>MEKTRPDYTSFNTVDEWLEAIKMGQYKESFANAGFTSFDVVSQMMMEDILRVGVTLAGHQKKILNSIQVMRAQMNQIQSVEV[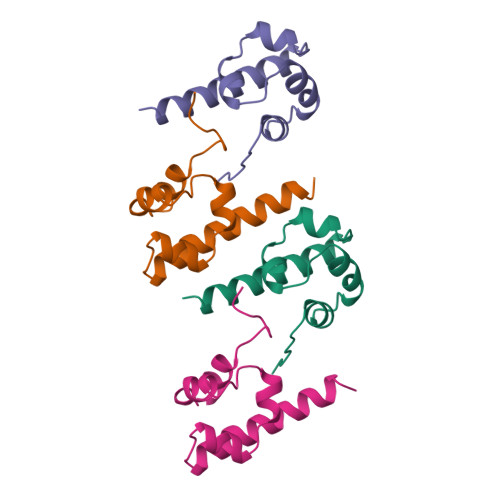8x]>[2x]CGC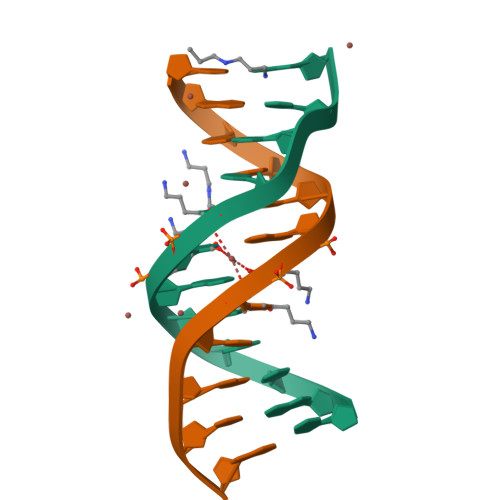GAAUUCGCG> SNAMSRGMSGLEDSSDLVVSPYVRMGGLTTDPVPTGGDDPHKVAMLGLTFDDVLLLPAASDVVPATADTSSQLTKKIRLKVPLVSSAMDTVTESRMAIAMARAGGMGVLHRNLPVAEQAGQVEMVKRSGGLLVGAAVGVGGDAWVRAMMLVDAGVDVLVVDTAHAHNRLVLDMVGKLKSEVGDRVEVVGGNVATRSAAAALVDAGADAVKVGVGPGSICTTRVVAGVGAPQITAILEAVAACRPAGVPVIADGGLQYSG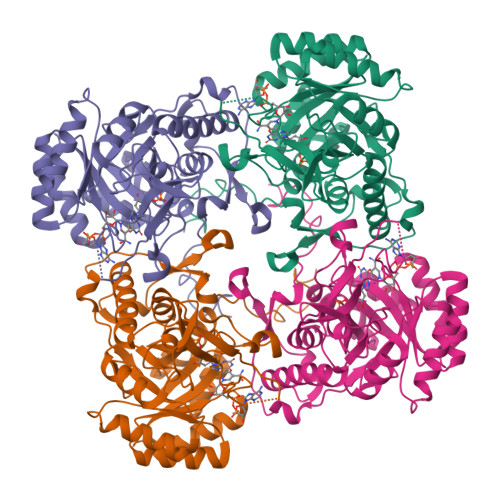DIAKALAAGASTAMLGSLLAGTAEAPGELIFVNGKQYKSYRGMGSLGAMRGRGGATSYSKDRYFADDALSEDKLVPEGIEGRVPFRGPLSSVIHQLTGGLRAAMGYTGSPTIEVLQQAQFVRITPAGLKESHPHDVAMTVEAPNYYAR> GGGRPTEIENINPNVYDRIKERVLTANEEDENVPDPFDKREIFDLIRNINDPEHPLTLEELHVVQEDLIRINDSQNSVHISFTPTIPHCSMATLIGLSIRVKLLRSLPPRFKV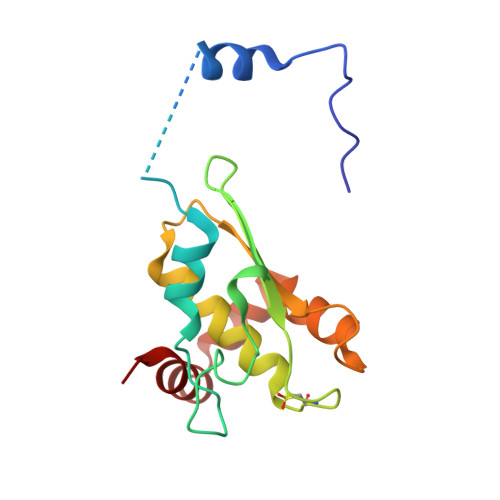TVEITPGTHASELAVNKQLADKERVAAALENNHLAEVINQCIAAKG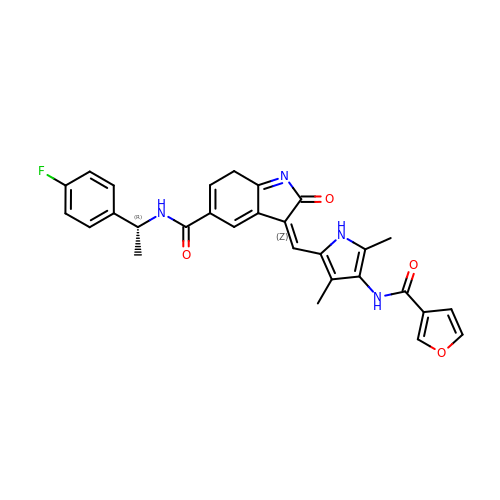(3Z)-N-[(1R)-1-(4-fluorophenyl)ethyl]-3-({4-[(furan-3-carbonyl)amino]-3,5-dimethyl-1H-pyrrol-2-yl}methylidene)-2-oxo-3,7-dihydro-2H-indole-5-carboxamide | C29 H25 F N4 O4 | DTUOQJZFJLHXLS-GEWRUKCFSA-N> SVPDVMVVG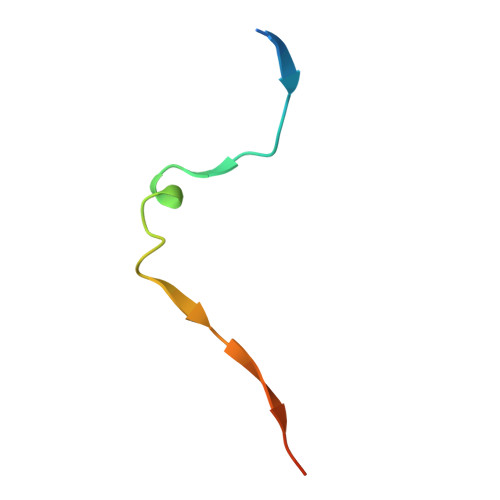EPTLMGGEFGDEDERLITRLENTQFDA Lysins (amidases, lysozymes/muramidases and peptidases) are such specialised bio-molecules. The term lysozyme, or muramidase, is broadly used to describe the enzymes that cleave the β-1,4-glycosidic bond between N-acetylglucosamine (NAG) and N-acetylmuramic acid (NAM) (or vice versa) in the carbohydrate backbone of peptidoglycan, Figure 1. Earlier reports had indicated the extraordinary stability of the digestive lysozyme from Opisthocomus hoazin at low pH, and the corresponding cDNA sequence (Genbank entry AAA73935.1) had been published. In addition, we have determined the crystal structure of the apo enzyme and of complexes with reaction products (chito-oligosaccharides). The structure presented here is the first to be determined for the avian upper-gut subset of GH22 lysozymes, and is, as expected, very similar overall to other C-type lysozymes.

As expected, OhLys has a typical GH22 lysozyme fold. The chain was traced from Glu1 through to Cys126, with a glycerol from the cryoprotectant, four Cl− ions and 200 water molecules. There are four disulphide bridges (Cys6–Cys126, Cys30–Cys114, Cys63–Cys79 and Cys75–Cys93) in the structure. The overall charge of OhLys differs somewhat from that of other C-type lysozymes. This increase in negative charge of OhLys is evident in the surface electrostatics of the enzyme. While the significance of this is not clear, it should be noted that the peptidoglycan substrate is also a charged molecule, and that peptidoglycan from different bacterial sources have different pI. So, charge interactions between the enzyme and the substrate at working pH are probably functionally important.

> EIIPRCELVKILREHGFEGFEGTTIADWICLVQHESDYNTEAYNNNGPSRDYGIFQINSKYWCNDGKTSGAVDGCHISCSELMTNDLEDDIKCAKKIARDAHGLTPWYGWKNHCEGRDLSSYVKGC>GSLVEEELDPFSLVADELSLLSNKLREMVLAEVPKLASAAEYFFKRGVQGKQFRSTILLLMATALDVRVPEALIGESTDIVTSELRVRQRGIAEITEMIHVASLLHDDVLDDADTRRGVGSLNVVMGNKMSVLAGDFLLSRACGALAALKNTEVVALLATAVEHLVTGETMEITSSTAARYSMDYYMQ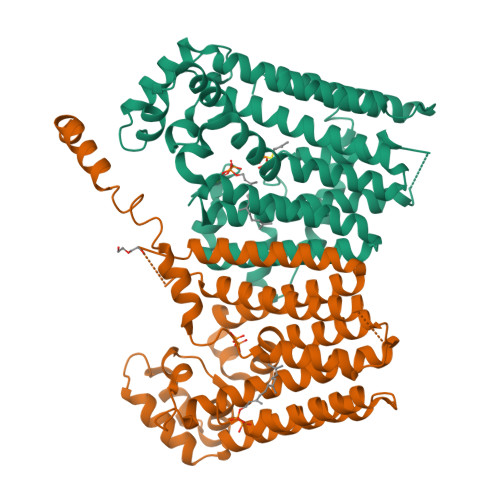KTYYKTASLISNSCKAVAVLTGQTAEVAVLAFEYGRNLGLAFQLIDDILDFTGTSASLGKGSLSDIRHGVITAPILFAMEEFPQLREVVDQVAADPRNVDIALEYLGKSKGIQRARELAMEHANLAAAAIGSLPETDNEDVKRSRRALIDLTHRVITRNK[8x]> MSLQMVTVGHNIALIQPGFSLMNFDGQVFFFGQKGWPKRSCPTGVFHFDIKQNHLKLKPAIFSKDSCYLPPLRYPATCSYKGSIDSDKHQYIIHGGKTPNNELSDKIYIMSVACKNNKKVTFRCTEKDLVGDVPEPRYGHSIDVVYSRGKSMGVLFGGRSYMPSTQRTTEKWNSVADCLPHVFLIDFEFGCATSYILPELQDGLSFHVSIARNDTVYILGGHSLASNIRPANLYRIRVDLPLGTPAVNCTVLPGGISVSSAILTQTNNDEFVIVGGYQLENQKRMVCSLVSLGDNT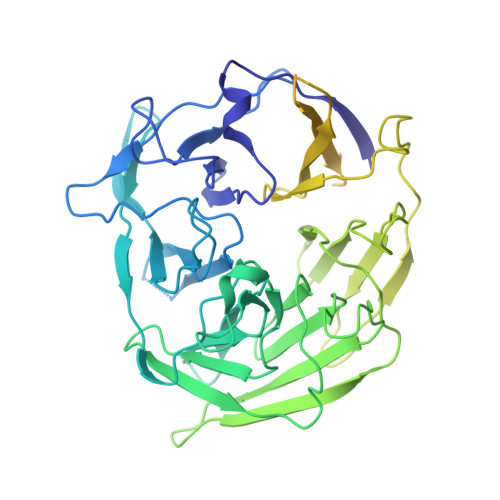IEISEMETPDWTSDIKHSKIWFGSNMGNGTIFLGIPGDNKQAMSEAFYFYTLRCSEEDLSEDQKIVSNSQTSTEDPGDSTPFEDSEEFCFSAEATSFDGDDEFDTYNEDDEDDESVTGYWITCCPTCDVDINTWVPFYSTELNKPAMIYCSHGDGHWVHAQCMDLEERTLIHLSEGSNKYYCNEHVQIARALQAPKRNPPLQKPPMKSLHKKGSGKVLTPAKKS> RSNESTSIRVAVEKVDQLINLVGELVITQSMLAQRSSELDPVNHGDLITSMGQLQRNARDLQESVMSIRMMPMEYVFSRYPRLVRDLAGKLGKQVELTLVGSSTELDKSLIERIIDPLTHLVRNSLDHGIELPEKRLAAGKNSVGNLILSAEHQGGNICIEVTDDGAGLNRERILAKAASQGLTVSENMSDDEVAMLIFAPGFSTAEQVTDVSGRGVGMDVVKRNIQKMGGHVEIQSKQGTGTTIRILLPLTLAILDGMSVRVADEVFILPLNAVMESLQPREADLHPLAGGERVLEVRGEYLPIVELWKVFNVAGAKTEATQGIVVILQ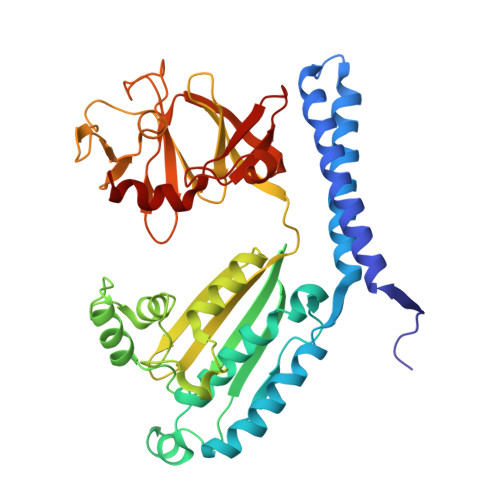SGGRRYALLVDQLIGQHQVVVKNLESNYRKVPGISAATILGDGSVALIVDVSALQAINREQ4-[5-(4-fluorophenyl)-3-(pyridin-4-ylmethyl)imidazol-4-yl]-1~{H}-pyrrolo[2,3-b]pyridine 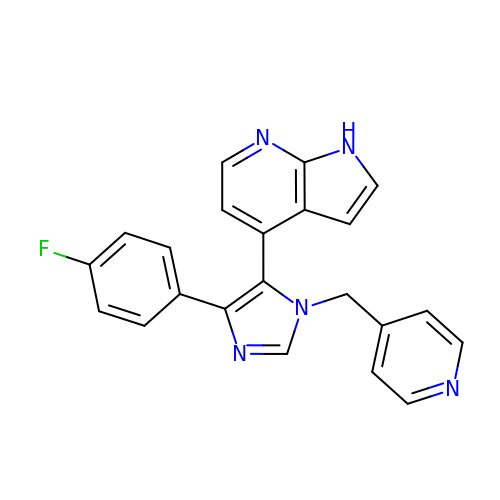| C22 H16 F N5 | RJSIBZBOEOZVIR-UHFFFAOYSA-N~{N}4-[3-(4-fluorophenyl)propyl]-6-(trifluoromethyl)pyridine-2,4-diamine | C15 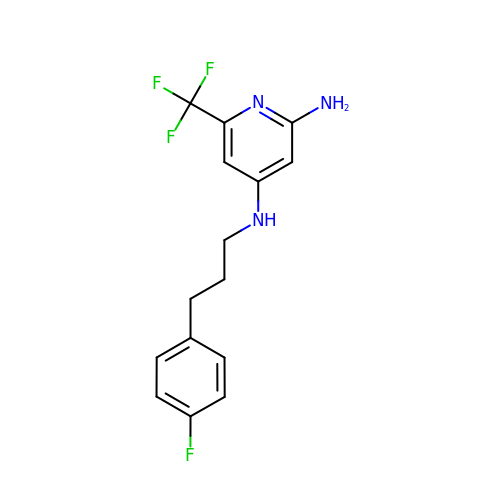H15 F4 N3 | AUZFKJZRALGBMB-UHFFFAOYSA-N> MTEQEIFEKVKAVIADKLQVEPEK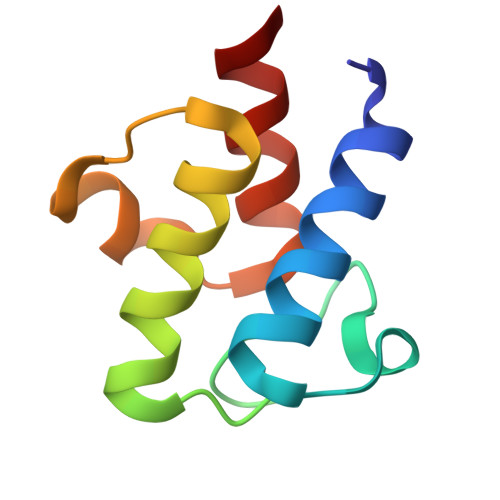VTLEARFIEDLGADSLDTVELIMGLEDEFGLEISDEEAEKIRTVKDAVEYIKAKLG methyl 3-(methylsulfonylamino)benzoate | C9 H11 N O4 S 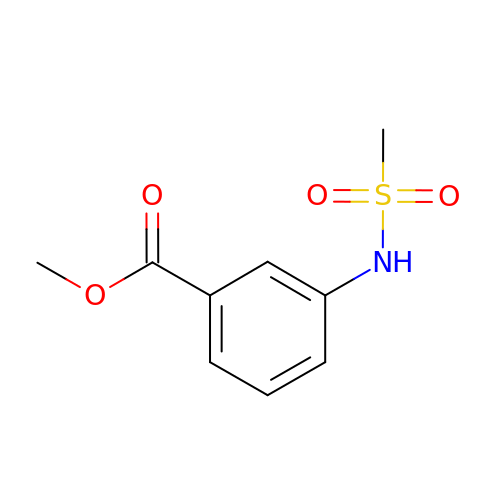| UQIOKJVVJMHUTP-UHFFFAOYSA-N> GSMSSFLGKWKLSESHNFDAVMSKLGVSWATRQIGNTVTPTVTFTMDGDKMTMLTESTFKNLS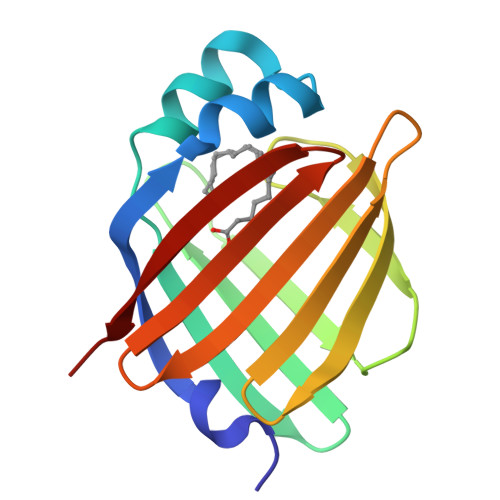CTFKFGEEFDEKTSDGRNVKSVVEKNSESKLTQTQVDPKNTTVIVREVDGDTMKTTVTVGDVTAIRNYKRLS>GSLSKVEESQLNEKENKNVADGLAWSYYFGYLKFVLPELEKQIEKTSKFRSKEKFVKKMFILIPSNCFWDDKIPGSDYDPQNRITFEGNTEPLEKTRGGVFLRHYKHSVYEIKDGENEPWFCIMEYATPLLTLYDMSVAQPGELSREERDAQVVVFLRKLQDILEGDRA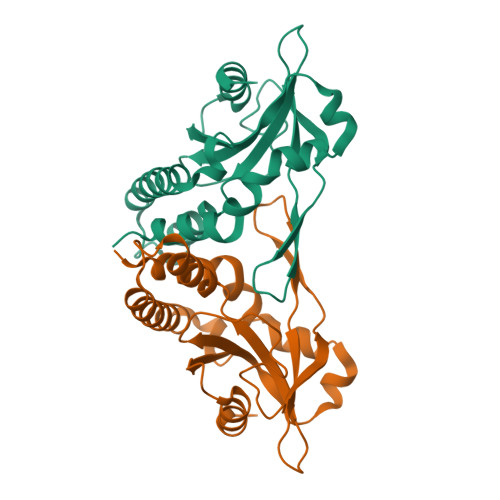CQGKYELVTFSPDRDLADVMLRKLKDSELEIGG[2x]>MDYLFKLLLIGDSGVGKTCVLFRFSEDAFNSTFISTIG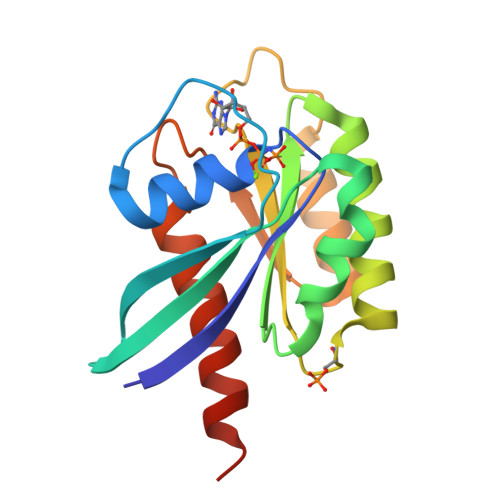IDFKIRTIELDGKRIKLQIWDTAGQERFRTITTAYYRGAMGIMLVYDITNEKSFDNIRNWIRNIEEHASADVEKMILGNKCDVNDKRQVSKERGEKLALDYGIKFMETSAKANINVENAFFTLARDIKAKMDKKHHHHHH[2x]Middle East respiratory syndrome coronavirus (MERS-CoV) and the pangolin MERS-like coronavirus MjHKU4r-CoV-1 employ dipeptidyl peptidase 4 (DPP4) as an entry receptor. To understand the mechanism of MjHKU4r-CoV-1 entry into cells, we determined the crystal structures of the receptor binding domain (RBD) of MjHKU4r-CoV-1 spike protein bound to human DPP4 (hDPP4) and Malayan pangolin DPP4 (MjDPP4), respectively. MjHKU4r-CoV-1 RBD is composed of a core structure and an external domain. The structure of hDPP4 or MjDPP4 consists of a α/β hydrolase domain and an eight-bladed β propeller domain. Both DPP4 receptors bind to MjHKU4r-CoV-1 RBM via blades IV and V of their β propeller domains, in agreement with the complex structures of MERS-CoV RBD-hDPP4 and Ty-BatCoV-HKU4 RBD-hDPP4 solved previously.

For the MjHKU4r-RBD and MjDPP4 complex, crystals were obtained in 0.1 M Ammonium tartrate dibasic (pH 7.0) and 12% (wt/vol) PEG 3350. The two MjHKU4r-CoV-1 RBD-MjDPP4 in the ASU are almost identical, with a RMSD of 0.335 Å over 936 aligned Cα atoms. However, when hDPP4 and MjDPP4 are superimposed, there is a 4.8° tilting angle between the respective MjHKU4r-CoV-1 RBDs bound to them. The larger BSA between MjHKUr-CoV-1 RBD and MjDPP4 also results in slight changes of the contact residues on the binding interface. Compared to the MjHKUr-CoV-1 RBD-hDPP4 complex, there are extra contacts between MjHKUr-CoV-1 RBD and MjDPP4, which involve residues M460, S511, Y525, A567 and L569 of viral RBD, and G296, D331, P333, S339 and R342 of MjDPP4. As MjHKU4r-CoV-1 RBD is orientated differently on hDPP4 and MjDPP4, there are also interactions specific to each complex. The RBD residue D471 only forms a salt bridge interaction with hDPP4 R336. In contrast, E544 contacts K267 of MjDPP4 via a salt bridge. Unexpectedly, although D471 is not in direct contact with residues in MjDPP4, D471A mutation showed a 10-fold reduction in affinity of MjHKU4r-CoV-1 RBD to MjDPP4, which is likely contributed by allosteric effects. The side chain of D471 forms a network of hydrogen bond interactions, either directly, or through water molecules, with Y506 and Q508 of MjHKUr-CoV-1 RBD, both of which contact MjDPP4.

>[2x]DKECDFTPMLVGVPPQVYNFKRLVFTNCNYNLTKLLSLFMVNEFSCNGISPDAIARGCYSSLTVDYFAYPLSMRSYIQPGSAGDISLYNYKQSFANPTCRVLATAPANLTLTKPSAYGYFQKCSRVSGEHNSVETPLYINPGEYSICRSFSPYGFSEDGEVFRRQLTQYEGGGILVGVGAKLAMTDKLEMGFIISVQYGTDTN;>[2x]RRTYTLTDYLKNTFRVKFYSLRWVSDHEYLYKQENNILLFNAEYGNSSIFLENSTFDEFGHSINDYSVSPDGQFILFEYNYVKKWRHSYTASYDIYDLHKRQLITEERIPNNTQWITWSPVGHKLAYVWHNDIYIKKEPNLQSQRITWTGKEDVIYNGITDWVYEEEVFSAYSALWWSPNGTFLAYAQFNDTEVPLIEYSFYSDESLQYPKTMQVPYPKAGAANPTVKLFVVNTDSLNSTANATSVQVVPPASVLIGDHYLCDVTWVNEERISLQWLRRIQNYSVLAICDYDKPTGRWASHVRQQHIESSTTGWVGRFKPSEPHFTSDGNSFYKIISNKEGYKHICHFQVDRENCTFITKGVWEVIGIEALTSDDLYYISNEYKGMPGGRNLYKIQLNDHTKVTCLSCELNTERCQYYSVSFSKEAKYYQLRCSGPGLPLYTLHSSSNDKELRVLEDNSALDKMLQDVQMPSKKLDFIIWNGIKLWYQMILPPHFDKLKKYPLLIDVYAGPCSQKADTVFRLNWATYLASTEKIIVASFDGRGSGYQGDKILHAINRRLGTLEVEDQIEAARQFTNMGFVDEKRIAIWGWSYGGYVTSMVLGAGSGVFKCGIAVAPVSRWEYYDSVYTERYMGLPTPEDNLEHYRNSTVMSRAENFKQVEYLLIHGTADDNVHFQQSAQISKALVDAGVDFQAMWYTDEDHGIASSTAHQHIYTHMSHFIKQCFSLPE>[2x]GMHAIKAVVFDLYGTLYDVYSVRTSCERIFPGQGEMV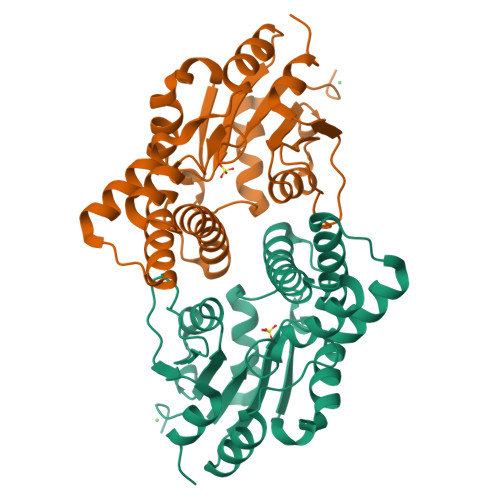SKMWRQKQLEYTWMRTLMGQYQDFESATLDALRYTCGSLGLALDADGEAHLCSEYLSLTPFADVPQALQQLRAAGLKTAILSNGSRHSIRQVVGNSGLTNSFDHLISVDEVRLFKPHQKVYELAMDTLHLGESEILFVSCNSWDATGAKYFGYPVCWINRSNGVFDQLGVVPDIVVSDVGVLASRFSPVDEAA>GVQPLATQCFQLSNMFNPQTEEEVGWDTEIKDDVIEECNKHGGVIHIYVDKNSAQGNVYVKCPSIAAAIAAVNALHGRWFAGKMITAAYVPLPTYHNLFPDSMTAT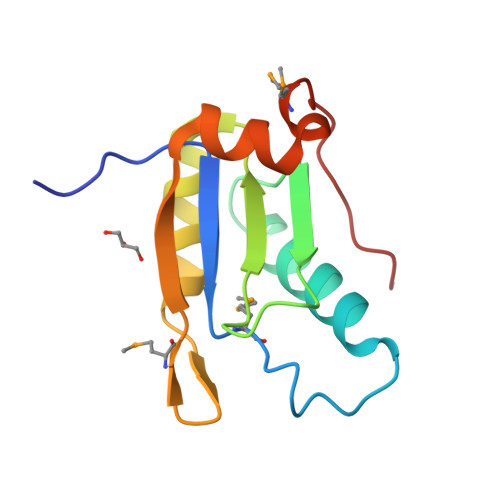QLLVPSRR[2x]>MASMGTLAFDEYGRPFLIIKDQDRKSRLMGLEALKSHIMAAKAVANTMRTSLGPNGLDKMMVDKDGDVTVTNDGATILSMMDVDHQIAKLMVELSKSQDDEIGDGTTGVVVLAGALLEEAEQLLDRGIHPIRIADGYEQAARVAIERLDKISDSVLVDIKDTEPLIQTAKTTLGSKVVNSCHRQMAEIAVNAVLTVADMERRDVDFELIKVEGKVGGRLEDTKLIKGVIVDKDFSHPQMPKKVEDAKIAILTCPFEPPKPKTKHKLDVTSVEDYKALQKYEKEKFEEMIQQIKETGANLAICQWGFDDEANHLLLQNNLPAVRWVGGPEIELIAIATGGRIVPRFSELTAEKLGFAGLVQEISFGTTKDKMLVIEQCKNSRAVTIFIRGGNKMIIEEAKRSLHDALCVIRNLIRDNRVVYGGGAAEISCALAVSQEADKCPTLEQYAMRAFADALEVIPMALSENSGMNPIQTMTEVRARQVKEMNPALGIDCLHKGTNDMKQQHVIETLIGKKQQISLATQMVRMILKIDDIRKPGESEE[4x]

TRiC interacts with approximately 10% of the entire proteome and its function is absolutely essential for viability of the cell. The general subunit architecture of the CCTs subunits comprise three distinct domains: an equatorial domain that includes the nucleotide-binding site, an apical domain involved in substrate binding, and an intermediate domain that connects the equatorial and apical domains via two hinge regions. The CCT5 homo-oligomeric complex has the two back-to-back rings of eight subunits similar to the full human TRiC complex. Moreover, the human CCT5 homo-oligomeric complex is able to hydrolyze ATP and refold misfolded protein substrates.

A mutation in human CCT5 subunit at position 147 that replaces a histidine with an arginine residue has been implicated in hereditary sensory neuropathy, which is a class of disorder marked by degeneration of the nerve fibers in the sensory periphery neurons. Sergeeva and collaborators showed the CCT5-H147R mutant has reduced folding activity compared to CCT5-WT against human γD-crystallin and actin substrates. However, biochemical analysis of CCT5-H147R showed that it was still able to hydrolyze ATP and also refold protein substrates. The human CCT5 and CCT5-H147R subunits were solved at 3.5 Å and 3.6 Å resolution, respectively. Our crystal structure of the CCT5-H147R mutant shows the same double homo-octameric ring arrangement as CCT5-WT indicating that the mutation does not affect the oligomeric assembly capability of the homo-octameric ring of the CCT5-H147R subunit. The structure also shows that the Arg147 residue is not positioned in a way that would disrupt the inter-ring or intra-ring interfaces, therefore it is unlikely that the mutation would impair the oligomeric assembly of the full TRiC complex containing the CCT5-H147R subunit. In addition, the CCT5-H147R structure was solved in complex with the nucleotide ADP showing the mutant still can bind nucleotide like the wild-type CCT5. The electron density map for CCT5-H147R demonstrates clear density for the side chain of Arg147, and shows that it is positioned to make a hydrogen bond between the NE atom of Arg147 located on helix-5 and the main carbonyl group of Ser428 located at helix-13 of the equatorial domain. Changes in contacts between structural elements in the complex could have an impact on the flexibility within the equatorial domain, thus modulating the function of a particular subunit. Since TRiC is a highly allosteric molecular machine, the CCT5-H147R point mutation could have an impact on the function of the entire complex by changing cooperativity within the complex.> MTTTVGLICDDAVILATDKRASLGNLVADKEAKKLYKIDDYIAMTIAGSVGDAQAIVRLLIAEAKLYKMRTGRNIPPLACATLLSN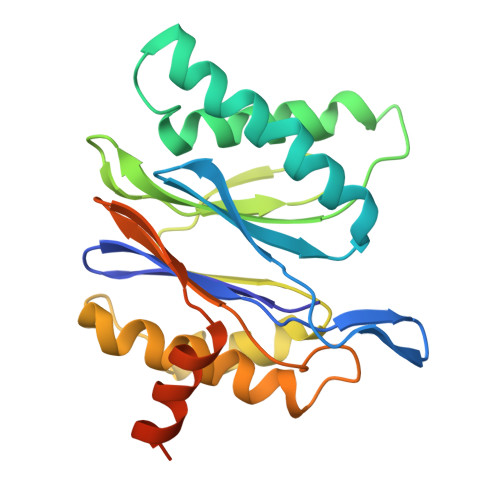ILHSSRMFPFLTQIIIGGYDLLEGAKLFSLDPLGGMNEEKTFTATGSGSPIAYGVLEAGYDRDMSVEEGIKLALNALKSAMERDTFSGNGISLAVITKDGVKIFEDEEIEKILDSMKAKPKKKTTKRSRRKSK> DYKDDDDKAEVKKIPTMIEGFDDISHGGLPQGATTLVSGTSGTGKTLFAVQFLYNGITIFNEPGIFVTFEESPQDIIKNALSFGWNLQSLIDQGKLFILDASPDPD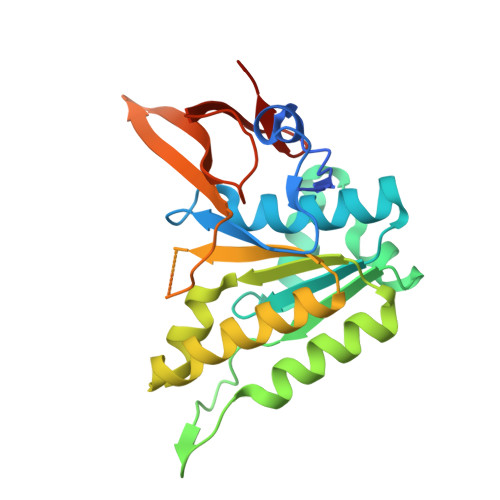GQEVAGDFDLSALIERIQYAIRKYKATRVSIDSVTAVFQQYDAASVVRREIFRLAFRLAQLGVTTIMTTERVDEYGPVARFGVEEFVSDNVVILRNVLEGERRRRTVEILKLRGTTHMKGEYPFTINNGINIFDYKDDDDK> GSAMALKVGVVGNPPFVFYGEGKNAAFTGISLDVWRAVAESQKWNSEYVRQNSISAGITAVAEG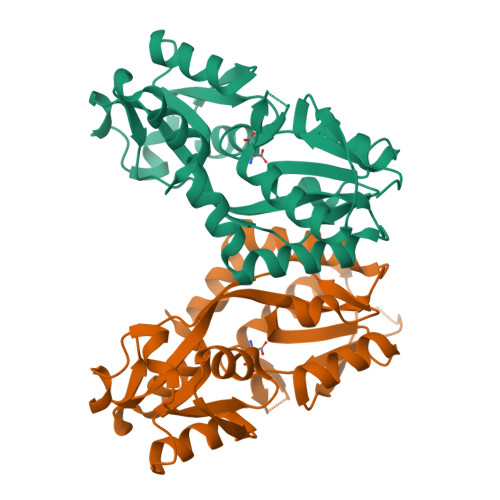ELDILIGPISVTPERAAIEGITFTQPYFSSGIGLLIPGTATPLFRSVGDLKNKEVAVVRDTTAVDWANFYQADVRETNNLTAAITLLQKKQVEAVMFDRPALIYYTRQNPNLNLEVTEIRVSLEPYGFVLKENSPLQKTINVEMLNLLYSRVIAEFTERWLGPGIEENQ> EDDLYRQSLEIISRYLREQATGSKDSKPLGEAGAAGRRALETLRRVGDGVQRNHETAFQGMLRKLDIKNEDDVKSLSRVMIHVFSDGVTNWGRIVTLISFGAFVAKHLKTINQESCIEPLAESITDVLVRTKRDWL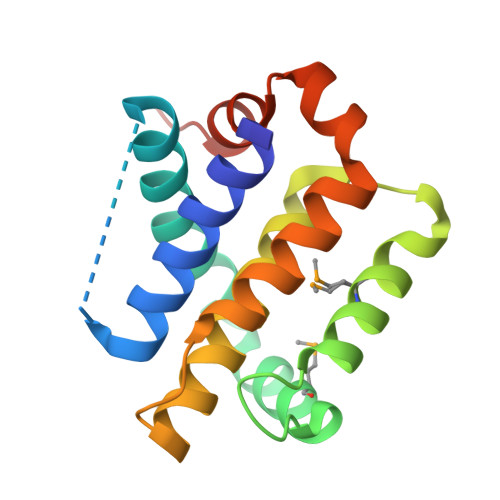VKQRGWDGFVEFFHVEDLEGG> TVPGATTTSSAATETMENVKKCKNFLSTLIKLASSGKQSTETAANVKELVQNLLDGKIEAEDFTSRLYRELN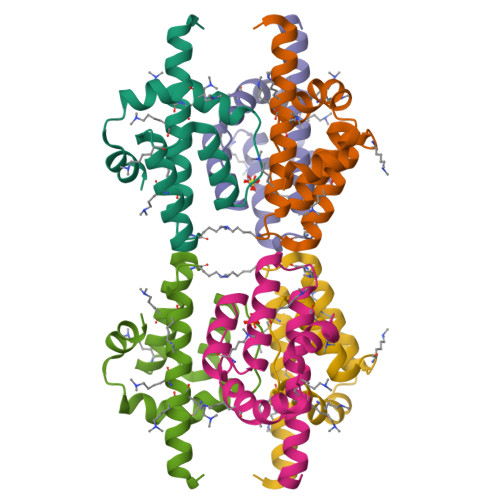SSPQPYLVPFLKRSLPALRQLTPDSAAFIQQSQQQPPPPTSQ> MSSFHATTIFAV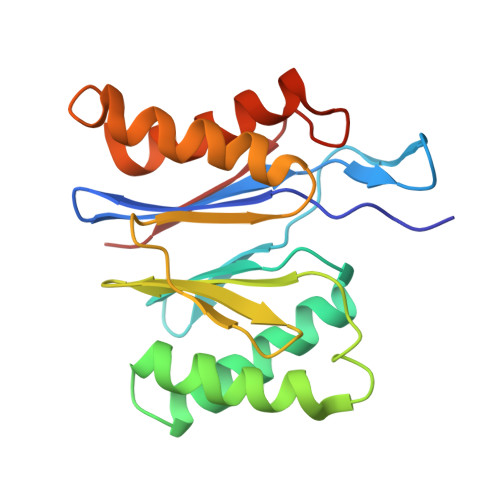QHKGRSAMSGDGQVTFGQAVVMKHTARKVRKLFNGKVLAGFAGSVADAFTLFEKFEAKLEEYNGNLKRAAVELAKEWRSDKVLRKLEAMLIVMNQDTLLLVSGTGEVIEPDDGILAIGSGGNYALAAGRALKKHAGESMSASEIARAALETAGEICVYTNDQIILEELE>[2x]TGRQEVRAESQFPGTRRPVSATIPGNFAAYHELWR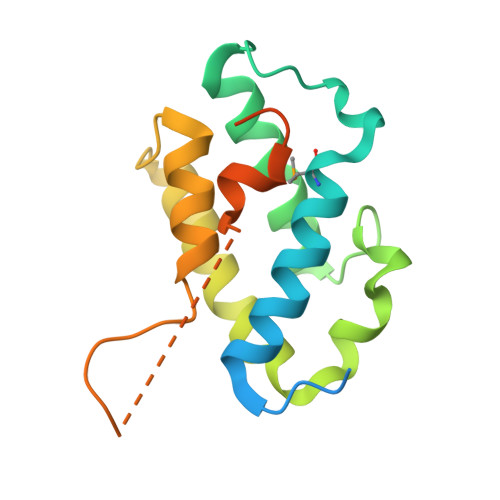NAFQEIMNDPRHQLHRNDVEYKKIHAIRTVLDDYTKGGNTWWAKFRRIFTFHWNRHHVKVVDDIVKEIDAGNYTTSRALVDRLDNLAISLGSKLNPKGTLKEQIGFIKIQEQNPVEEIENLSRPNLT[(2R)-2-{2-[hydroxy(methyl)amino]-2-oxoethyl}-5-(naphthalen-1-yl)pentyl]phosphonic acid 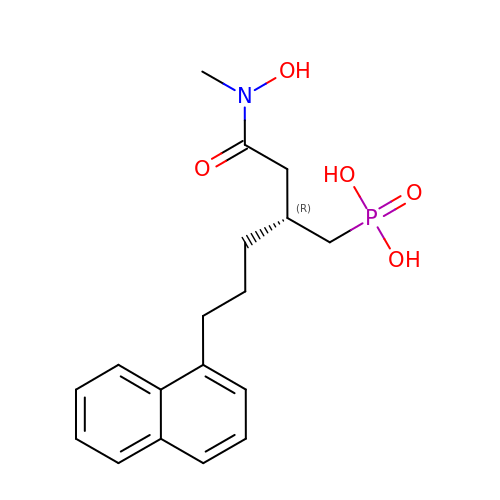| C18 H24 N O5 P | HUBGFLNAUJJVOG-CQSZACIVSA-N>[6x]GPMVTVTYDPSNAPSFQQEIANAAQIWNSSVRNVQLRAGGNADFSYYEGNDSRGSYAQTDGHGRGYIFLDYQQNQQYDSTRVTAHETGHVLGLPDHYQGPCSELMSGGGPGPSCTNPYPNAQERSRVNALWANG;>GSAHGPSAM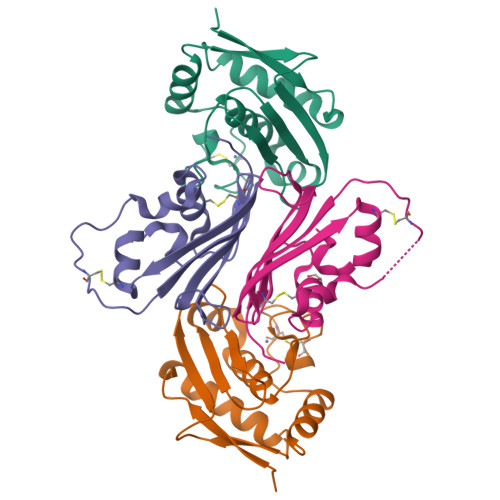VFTVIQGSGEPTDTVLRATTLSCAYTAEGTHPAPRAACDALNATDGELNRLLAAPDPSLVCPMYFDPVTVTADGVLNGRRVAWKHTFSNTCVMSANLNSNPVYAF[6x]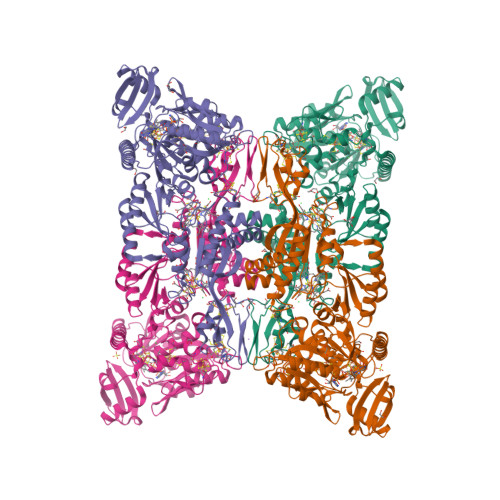>[16x]MYEWKLNDIVDNGICAKCGTCTVVCPNGILTFEDRPKLTEECLRKGNGMCFEVCPRVSSGKYQIKIREKFKEEYYYGKGDVEGQDGGVVTTFLKYLLKNKKIDGAIVVGDECWKPVSLIVQNEEDLMNTTKSKYTVSTLEALKTAGEMGLEKVAVVGLPCQINGLRKLQYFQYLAKHDGELGKNGKPVKLPKIEYLIGLLCTEKFEYDELKETLAKYNINMDDVEKFDIKKGKLLVYVNGEEHKIPLKEIELSAGCKMCRDFDAEMADVSVGCVGSPDGYSTVIIRTEKGEEIKNAIELKEGVNLEAIEKLRDLKLNRFKKEVERRKAEDEKVSFYWTADYGGVGKRADGTYFIRIRAKPAGWYSIDEAREILEIAEKYDGKIKMTNRGAFEIHGISGFDVEAMVLELMEKGFITGSEGPLVRATLACPGEGNCGSGLINTTELCKILEDNFKEHPAPYKFKIAISGCPNKCVRPQIHDIGIAGVKFPVVNEENCNGCGRCAEVCKIEAIDIRGETSYTNYNVCIGCGKCIKACPNEGRDVKEEGFMVYVGGKTGREVIEGVSMKLMSVEEILNLIDKVLIVYHKYAKKPQRERLAAVMARIGKGKFLEEVKELMEQN> QIEQQSPWEFQGSEVWQQHRYQSPRACRLENLRAQDPVRRAEAEAGFTEVWDQDNDEFQCAGVNMIRHTIRPKGLLLPGFSNAPKLIFVAQGFGIRGIAIPGCAETYQTDLRRSQSAGSAFKDQHQKIRPFREG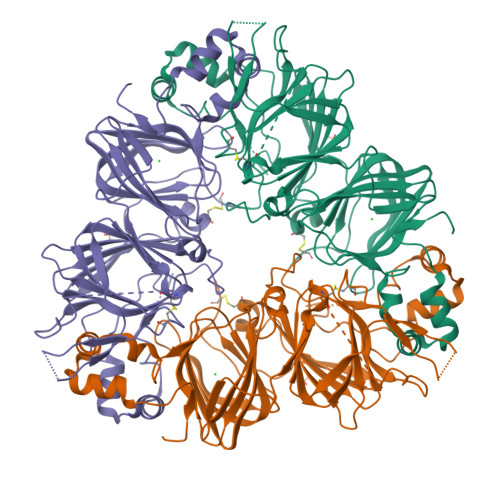DLLVVPAGVSHWMYNRGQSDLVLIVFADTRNVANQIDPYLRKFYLAGRPEQVERGVEEWERSSRKGSSGEKSGNIFSGFADEFLEEAFQIDGGLVRKLKGEDDERDRIVQVDEDFEVLLPEKDEEERSRGRYIESESESENGLEETICTLRLKQNIGRSERADVFNPRGGRISTANYHTLPILRQVRLSAERGVLYSNAMVAPHYTVNSHSVMYATRGNARVQVVDNFGQSVFDGEVREGQVLMIPQNFVVIKRASDRGFEWIAFKTNDNAITNLLAGRVSQMRMLPLGVLSNMYRISREEAQRLKYGQQEMRVLSPGRSQGRRE> RTPEMPVLENRAAQGDITAPGGARRLTGDQTAALRDSLSDKPAKNIILLIGDGMGDSEITAARNYAEGAGGFFKGIDALPLTGQYTHYALNKKTGKPDYVTDSAASATAWSTGVKTYNGALGVDIHEKDHPTILEMAKAAGLATGNVSTAELQDATPAALVAHVTSRKCYGPSATSEKCPGNALEKGGKGSITEQLLNARADVTLGGGAKTFAETATAGEWQGKTLREQAQARGYQLVSDAASLNSVTEANQQKPLLGLFADGNMPVRWLGPK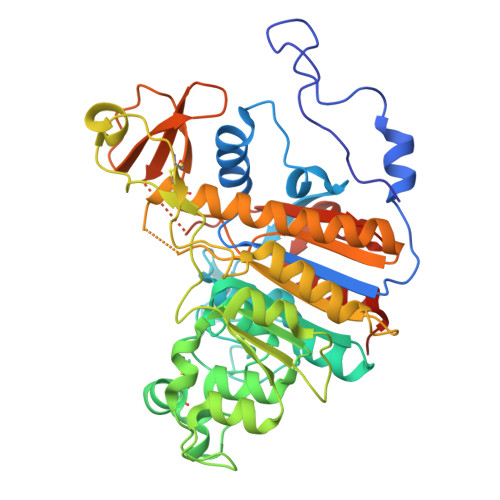ATYHGNIDKPAVTCTPNPQRNDSVPTLAQMTDKAIELLSKNEKGFFLQVEGASIDKQDHAANPCGQIGETVDLDEAVQRALEFAKKEGNTLVIVTADHAHASQIVAPDTKAPGLTQALNTKDGAVMVMSYGNSEEDSQEHTGSQLRIAAYGPHAANVVGLTDQTDLFYTMKAALGLKLEEEEEEE> SKASVKITPLGGLGEIGGNMMVIETPKSAIVIDAGMSFPKEGLFGVDILIPDFSYLHQIKDKIAGIIITHAHEDHIGATPYLFKELQFPLYGTPLSLGLIGSKFDEHGLKKYRSYFKIVEKRCPISVGEFIIEWIHITHSIIDSSALAIQTKAGTIIHTGDFKIDHTPVDNLPTDLYRLAHYGEKGVMLLLSDSTNSHKSGTTPSESTIAPAFDTLFKEAQGRVIMSTFSS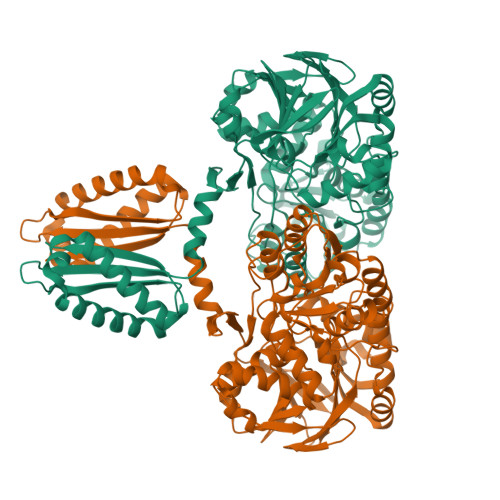NIHRVYQAIQYGIKYNRKIAVIGRSMEKNLDIARELGYIHLPYQSFIEANEVAKYPDNEILIVTTGSQGETMSALYRMATDEHRHISIKPNDLVIISAKAIPGNEASVSAVLNFLIKKEAKVAYQEFDNIHVSGHAAQEEQKLMLRLIKPKFFLPVHGEYNHVARHKQTAISCGVPEKNIYLMEDGDQVEVGPAFIKKVGTIKSGKSYVDNQSNLSIDTSIVQQREEVASAGVFVATIFVNKNKQALLESSQFSSLGLVGFKDEKPLIKEIQGGLEVLLKSSNAEILNNPKKLEDHTRNFIRKALFKKFRKYPAIICHAHSF> ENSHNKARTSPYPGSKVERSQVPNEKVGWLVEWQDY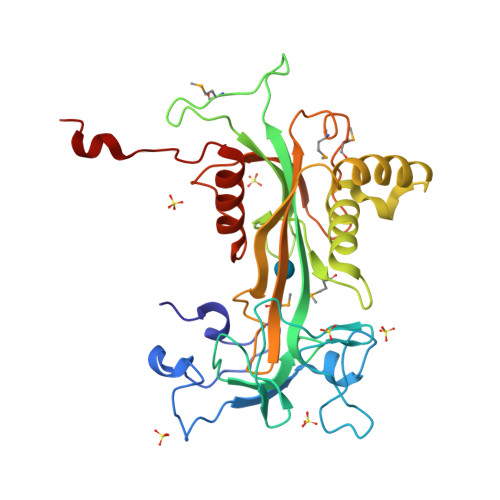KPVEYTAVSVLAGPRWADPQISESNFSPKFNEKDGHVERKSKNGLYEIENGRPRNPAGRTGLVGRGLLGRWGPNHAADPIITRWKRDSSGNKIMHPVSGKHILQFVAIKRKDCGEWAIPGGMVDPGEKISATLKREFGEEALNSLQKTSAEKREIEEKLHKLFSQDHLVIYKGYVDDPRNTDNAWMETEAVNYHDETGEIMDNLMLEAGDDAGKVKWVDINDKLKLYASHSQFIKLVAEKRDAHWSEDSEADCHAL> AEPPLVFEPVTLESLRQEAGFQAVGAAQIAELDTLRAAHAAERTSVQKTQNAAIDKLIKGKSKDDIRNDANIKNSINDQTKQWTDMIARHRKEEWDMLRQHVQDSQDAMKALMLTVQAAQIKQLEDRHARDIKDLNAKQAKMSADTAKEVQNDKTLKTKNEKDRRLREKRQNNVKRFMEEKKQIGVKQGRAMEKLKLAHSKQIEEFSTDVQKLMDMYKIEEE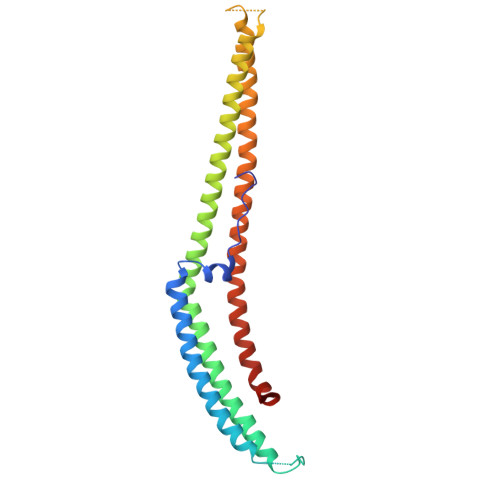AYKTQGKTEFYA> GEVASVPLTNYLDSQYFGKIYLGTPPQEFTVLFDTGSSDFWVPSIYCKSNACKNHQRFDPRKSSTFQNLGKPLSIHYGTGSMQGILGYDTVTVSNIVDIQQTVGLSTQEPGDVFTYAEFD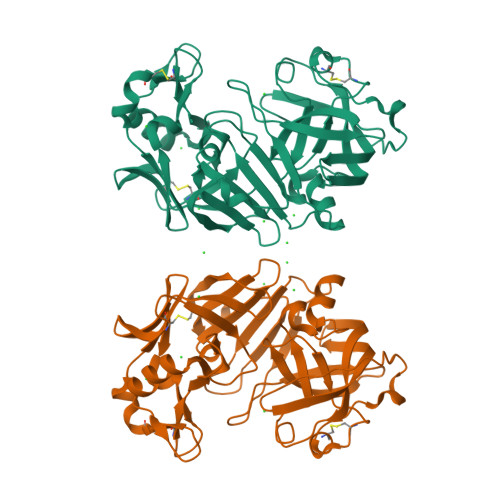GILGMAYPSLASEYSIPVFDNMMNRHLVAQDLFSVYMDRNGQESMLTLGAIDPSYYTGSLHWVPVTVQQYWQFTVDSVTISGVVVACEGGCQAILDTGTSKLVGPSSDILNIQQAIGATQNQYGEFDIDCDNLSYMPTVVFEINGKMYPLTPSAYTSQDQGFCTSGFQSENHSQKWILGDVFIREYYSVFDRANNLVGLAKAI>[4x]MLKVIQSPGKYLQGPDASTLFGAYAKNLAESFFVIADDFVMKLAGDKVLNGLHSHDISLHAERFNGECSHVEIRRLIAILKQHGCRGVVGVGGGKTLDTAKAIGYYQKLPVVVIPTIASTDAPTSALSVIYTEAGEFEEYLIYPKNPDMVVMDTAIIAKAPVRLLVSGMGDALSTWFEAKACYDARATSMAGGQSTEAALSL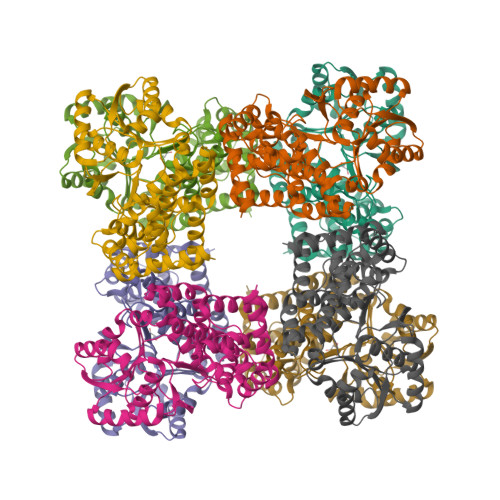ARLCYDTLLAEGEKARLAAQAGVVTDALERIIEANTYLSGIGFESSGLAAAHAIHNGFTILEECHHLYHGEKVAFGTLAQLVLQNSPMEEIETVLGFCEKVGLPVTLAQMGVKEGIDDKIAAVAKATCAEGETIHNMPFAVTPEQVHAAILTADLLGQQWLAR>MEFETIETKKEGNLFWITLNRPDKLNALNAKLLEELDRAVSQAESDPEIRVIIITGKGKAFCAGADITQFNQLTPAEAWKFSKKGREIMDKIEALSKPTIAMINGYALGGGLELALACDIRIAAEEAQLGLPEINLGIYPGYGGTQRLTRVIGKGRALEMMMTGDRIPGKDAEK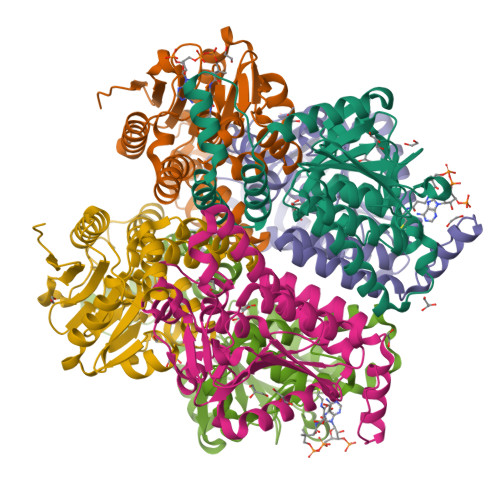YGLVNRVVPLANLEQETRKLAEKIAKKSPISLALIKEVVNRGLDSPLLSGLALESVGWGVVFSTEDKKEGVSAFLEKREPTFKGK[6x]> GSTGSRPILEVPESVTGPWRGDVNLPCTYDPLQGYTQVLVRWLVQRGSDPVTIFLRDSSGDHIQQARYQGRLHVSHRVPGDVSLQLSTLEMDDRSH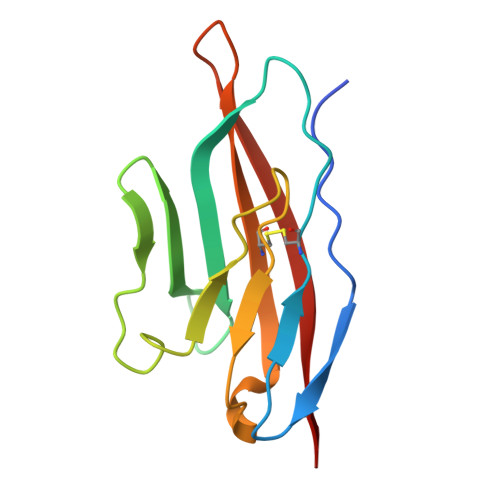YTCEVTWQTPDGNQVVRDRITELRVQK> MQVNRLPFFTNHFFDTYLLISEDTPVGSSVTQLLARDMDNDPLVFGVSGEEASRFFAVEPDTGVV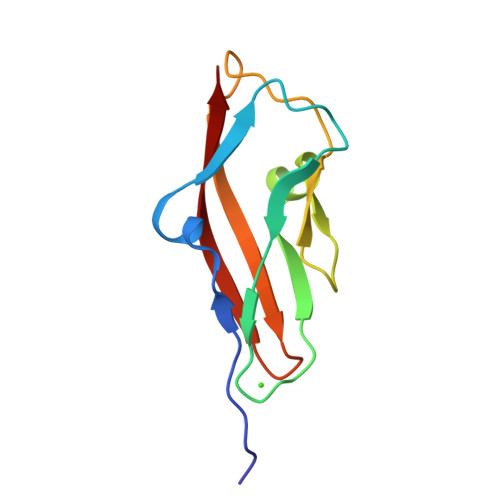WLRQPLDRETKSEFTVEFSVSDHQGVITRKVNIQVGD>[4x]GSHMASPSLWGDRFHSFSVDNQVAEKYAQEIETLKEQTSTMLSAACGTTLTEKL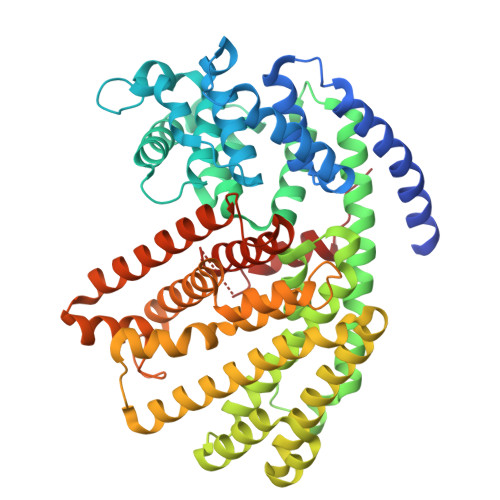NLIDIIERLGIAYHFEKQIEDMLDHIYRADPYFEAHEYNDLNTSSVQFRLLRQHGYNVSPNIFSRFQDANGKFKESLRSDIRGLLNLYEASHVRTHKEDILEEALVFSVGHLESAAPHLKSPLSKQVTHALEQSLHKSIPRVEIRYFISIYEEEEFKNDLLLRFAKLDYNLLQMLHKHELSEVSRWWKDLDFVTTLPYARDRAVECYFWTMGVYAEPQYSQARVMLAKTIAMISIVDDTFDAYGIVKELEVYTDAIQRWDISQIDRLPEYMKISYKALLDLYDDYEKELSKDGRSDVVHYAKERMKEIVRNYFIEAKWFIEGYMPSVSEYLSNALATSTYYLLTTTSYLGMKSATKEHFEWLATNPKILEANATLCRVVDDIATYEVEKGRGQIATGIECYMRDYGVSTEVAMEKFQEMADIAWKDVNEEILRPTPVSSEILTRILNLARIIDVTYKHNQDGYTHPEKVLKPHIIALVVDSIDI> MSQDTEVDMKEVELNELEPEKQPMNAASGAAMSLAGAEKNGLVKIKVAEDEAEAAAAAKFTGLSKEELLKVAGSPGWVRTRWALLLLFWLGWLGMLAGAVVIIVRAPRCRELPAQKWWHTGALYRIGDLQAFQGHGAGNLAGLKGRLDYLSSLKVK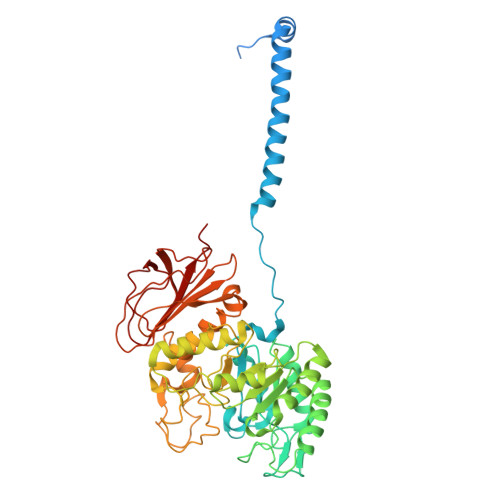GLVLGPIHKNQKDDVAQTDLLQIDPNFGSKEDFDSLLQSAKKKSIRVILDLTPNYRGENSWFSTQVDTVATKVKDALEFWLQAGVDGFQVRDIENLKDASSFLAEWQNITKGFSEDRLLIAGTNSSDLQQILSLLESNKDLLLTSSYLSDSGSTGEHTKSLVTQYLNATGNRWCSWSLSQARLLTSFLPAQLLRLYQLMLFTLPGTPVFSYGDEIGLDAAALPGQPMEAPVMLWDESSFPDIPGAVSANMTVKGQSEDPGSLLSLFRRLSDQRSKERSLLHGDFHAFSAGPGLFSYIRHWDQNERFLVVLNFGDVGLSAGLQASDLPASASLPAKADLLLSTQPGREEGSPLELERLKLEPHEGLLLRFPYAA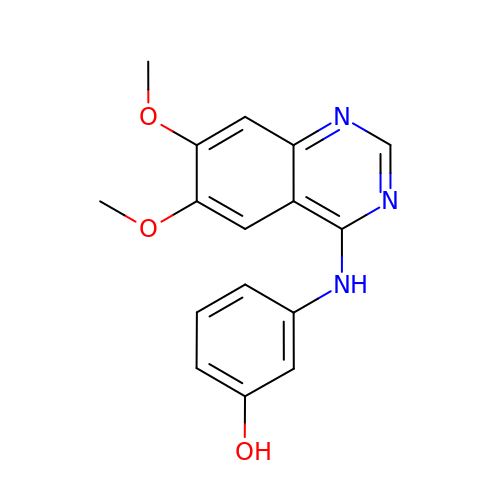4-[3-HYDROXYANILINO]-6,7-DIMETHOXYQUINAZOLINE | C16 H15 N3 O3 | BNDYIYYKEIXHNK-UHFFFAOYSA-N>[2x]MAVPETRPNHTIYINNLNEKIKKDELKKSLHAI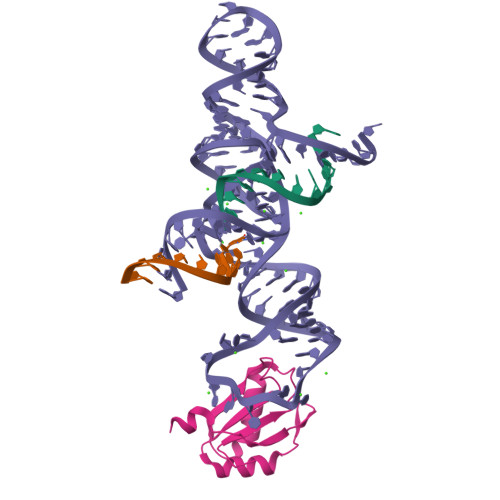FSRFGQILDILVSRSLKMRGQAFVIFKEVSSATNALRSMQGFPFYDKPMRIQYAKTDSDIIAKMKGT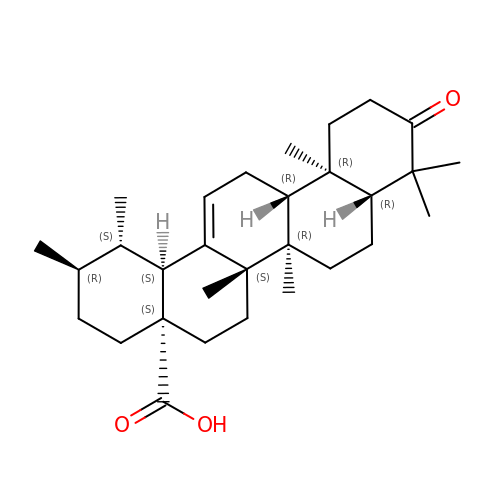(5beta)-3-oxours-12-en-28-oic acid | C30 H46 O3 | MUCRYNWJQNHDJH-OADIDDRXSA-N> IQGSLMDV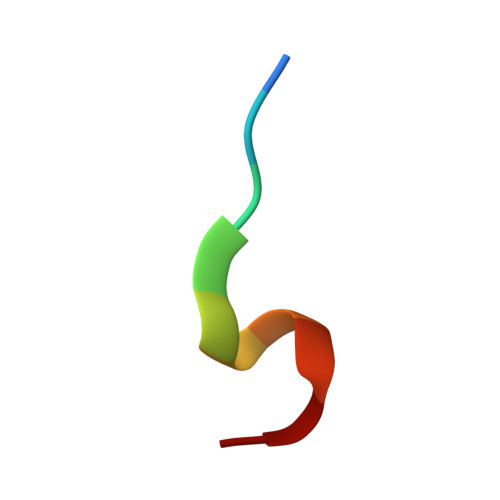GM>[2x]DNFQDLFTGAYHKYKVWRRQQMSFINKHERTLAIDGDYIYIVPPEGRIHWHDNV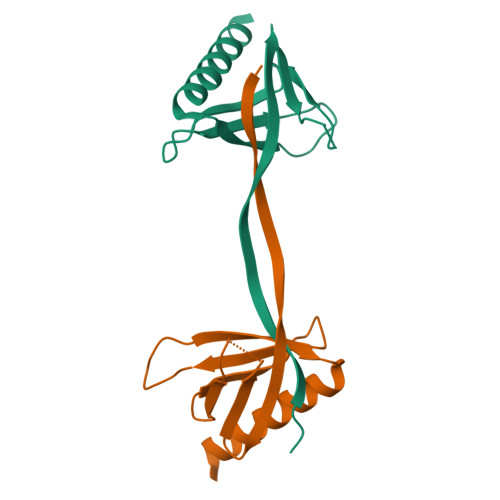KTKSLHISQVVLVKKSKRVPEHFKIFVRREGQDDIKRYYFEAVSGQECTEIVTRLQNLLSAYRMNHK>[6x]MCGRFLRRLLAEESRRSTPVGRL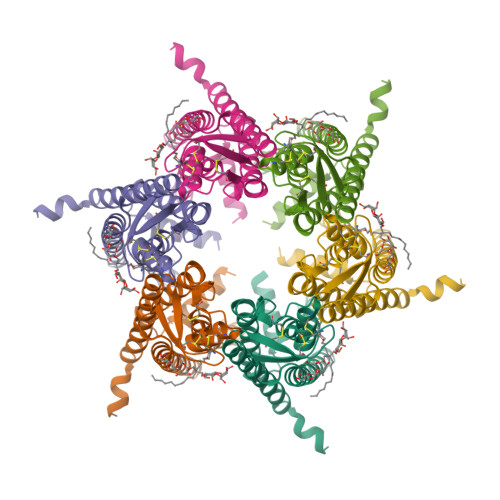LLPVLLGFRLVLLAASGPGVYGDEQSEFVCHTQQPGCKAACFDAFHPLSPLRFWVFQVILVAVPSALYMGFTLYHVIWHWELSGKGKEEETLIQGREGNTDVPGAGSLRLLWAYVAQLGARLVLEGAALGLQYHLYGFQMPSSFACRREPCLGSITCNLSRPSEKTIFLKTMFGVSGFCLLFTFLELVLLGLGRWWRTWKHKSSSSKYFLTSESTRRHKKATDSLPVVETKEQFQEAVPGRSLAQEKQRPVGPRDA>[6x]MAQIDFRKKINWHRRYRSPQGVKTEHEILRIFESDRGRIINSPAIRRLQQKTQVFPLERNAAVRTRLTHSMEVQQVGRYIAKEILSRLKELKLLEAYGLDELTGPFESIVEMSCLMHDIGNPPFGHFGEAAINDWFRQRLHPEDAESQPLTDDRCSVAALRLRDGEEPLNELRRKIRQDLCHFEGNAQGIRLVHTLMRMNLTWAQVGGILKYTRPAWWRGETPETHHYLMKKPGYY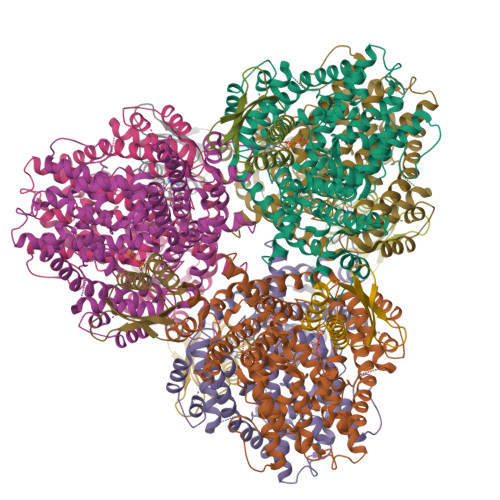LSEEAYIARLRKELNLALYSRFPLTWIMEAADDISYCVADLEDAVEKRIFTVEQLYHHLHEAWGQHEKGSLFSLVVENAWEKSRSNSLSRSTEDQFFMYLRVNTLNKLVPYAAQRFIDNLPAIFAGTFNHALLEDASECSDLLKLYKNVAVKHVFSHPDVERLELQGYRVISGLLEIYRPLLSLSLSDFTELVEKERVKRFPIESRLFHKLSTRHRLAYVEAVSKLPSDSPEFPLWEYYYRCRLLQDYISGMTDLYAWDEYRRLMAVEQ;>[6x]GSFTMGRLYSGNLAAFKAATNKLFQLDLAVIYDDWYDAYTRKDCIRLRIEDRSGNLIDTSTFYHHDEDVLFNMCTDWLNHMYDQLKDWK>[2x]SNATYQYNMNFEKLGKCIIINNKNFDKVTGMGVRNGTDKDAEALF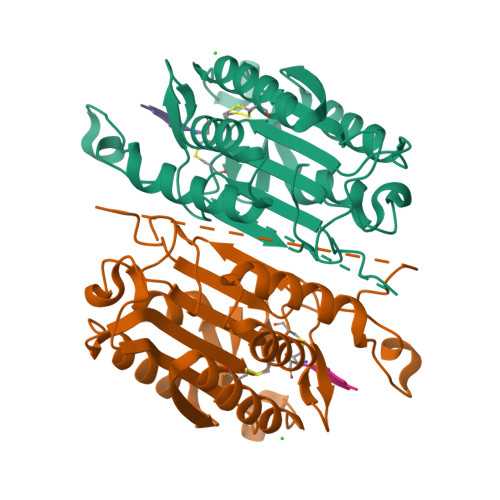KCFRSLGFDVIVYNDCSCAKMQDLLKKASEEDHTNAACFACILLSHGEENVIYGKDGVTPIKDLTAHFRGDRCKTLLEKPKLFFIQACRGTELDDGIQAASGPINDTDANPRYKIPVEADFLFAYSTVPGYYSWRSPGRGSWFVQALCSILEEHGKDLEIMQILTRVNDRVARHFESQSDDPHFHEKKQIPCVVSMLTKELYFSQ> MFNKSFGTPFGGGTGGFGTTSTFGQNTGFGTTSGGAFGTSAFGSSNNTGGLFGNSQTKPGGLFGTSSFSQPATSTSTGFGFGTSTGTANTLFGTASTGTSLFSSQNNAFAQNKPTGFGNFGTSTSSGGLFGTTNTTSNPFGSTSGSLFGPSSFTAAPTGTTIKFNPPTGTDTMVKAGVSTNISTKHQCITAMKEYESKSLEELRLEDYQANRKGPQNQVGAGTTTGLFGSSPATSSATGLFSSSTTNSGFAYGQNKTAFGTSTTGFGTNPGGLFGQQNQQTTSLFSKPFGQATTTQNTGFSFGNTSTIGQPSTNTMGLFGVTQASQPGGLFGTATNTSTGTAFGTGTGLFGQTNTGFGAVGSTLFGNNKLTTFGSSTTSAPSFGTTSGGLFGNKPTLTLGTNTNTSNFGFGTNTSGNSIFGSKPAPGTLGTGLGAGFGTALGAGQASLFGNNQPKIGGPLGTGAFGAPGFNTTTATLGFGAPQAPVALTDPNASAAQQAVLQQHINSLTYSPFGDSPLFRNPMSDPKKKEERLKPTNPAAQKALTTPTHYKLTPRPATRVRPKALQTTGTAKSHLFDGLDDDEPSLANGAFMPKKSIKKLVLKNLNNSNLFSPVNRDSENLASPSEYPENGERFSFLSKPVDENHQQDGDEDSLVSHFYTNPIAKPIPQTPESAGNKHSNSNSVDDTIVALNMRAALRNGLEGSSEETSFHDESLQDDREEIENNSYHMHPAGIILTKVGYYTIPSMDDLAKITNEKGECIVSDFTIGRKGYGSIYFEGDVNLTNLNLDDIVHIRRKEVVVYLDDNQKPPVGEGLNRKAEVTLDGVWPTDKTSRCLIKSPDRLADINYEGRLEAVSRKQGAQFKEYRPETGSWVFKVSHFSKYGLQDSDEEEEEHPSKTSTKKLKTAPLPPASQTTPLQMALNGKPAPPPQSQSPEVEQLGRVVELDSDMVDITQEPVLDTMLEESMPEDQEPVSASTHIASSLGINPHVLQIMKASLLTDEEDVDMALDQRFSRLPSKADTSQEICSPRLPISASHSSKTRSLVGGLLQSKFTSGAFLSPSVSVQECRTPRAASLMNIPSTSSWSVPPPLTSVFTMPSPAPEVPLKTVGTRRQLGLVPREKSVT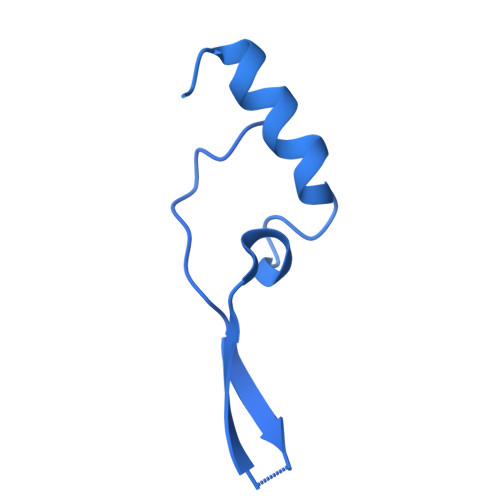YGKGKLLMDMALFMGRSFRVGWGPNWTLANSGEQLNGSHELENHQIADSMEFGFLPNPVAVKPLTESPFKVHLEKLSLRQRKPDEDMKLYQTPLELKLKHSTVHVDELCPLIVPNLGVAVIHDYADWVKEASGDLPEAQIVKHWSLTWTLCEALWGHLKELDSQLNEPREYIQILERRRAFSRWLSCTATPQIEEEVSLTQKNSPVEAVFSYLTGKRISEACSLAQQSGDHRLALLLSQFVGSQSVRELLTMQLVDWHQLQADSFIQDERLRIFALLAGKPVWQLSEKKQINVCSQLDWKRSLAIHLWYLLPPTASISRALSMYEEAFQNTSDSDRYACSPLPSYLEGSGCVIAEEQNSQTPLRDVCFHLLKLYSDRHYDLNQLLEPRSITADPLDYRLSWHLWEVLRALNYTHLSAQCEGVLQASYAGQLESEGLWEWAIFVLLHIDNSGIREKAVRELLTRHCQLLETPESWAKETFLTQKLRVPAKWIHEAKAVRAHMESDKHLEALCLFKAEHWNRCHKLIIRHLASDAIINENYDYLKGFLEDLAPPERSSLIQDWETSGLVYLDYIRVIEMLRHIQQVDCSGNDLEQLHIKVTSLCSRIEQIQCYSAKDRLAQSDMAKRVANLLRVVLSLHHPPDRTSDSTPDPQRVPLRLLAPHIGRLPMPEDYAMDELRSLTQSYLRELAVGSL> VVGGEDAKPGQFPWQVVLNGKVDAFCGGSIVNEKWIVTAAHCVETGVKITVVAGEHNIEETEHTEQKRNVIRIIPHHNYNAAINKYNHDIALLELDEPLVLNSYVTPICIA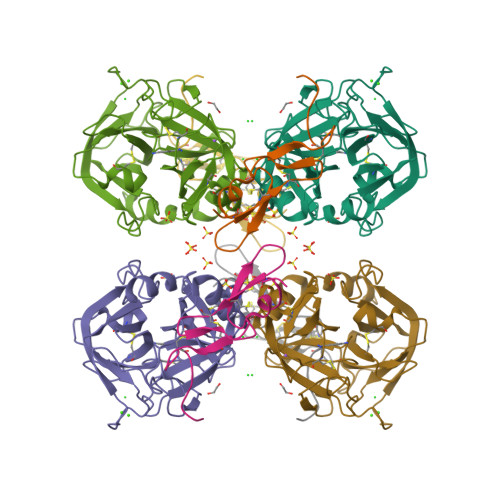DKEYTNIFLKFGSGYVSGWGRVFHKGRSALVLQYLRVPLVDRATCLRSTKFTIYNNMFCAGFHEGGRDSCQGDSGGPHVTEVEGTSFLTGIISWGEECAMKGKYGIYTKVSRYVNWIKEKTKLT;> MTCNIKNGRCEQFCKNSADNKVVCSCTEGYRLAENQKSCEPAVPFPCGRVSVSQ Aromatic residues cluster in the core of folded proteins, where they stabilize the structure through multiple interactions. NMR studies in the 1970s demonstrated that aromatic side chains can undergo ring flips—that is, 180° rotations of the χ2 dihedral angle (Cβ–Cγ axis)—even when engaged in stabilizing interactions in the hydrophobic core. Here we capture ring flipping events of a buried tyrosine residue in the SH3 domain of the JNK-interacting protein 1 (JIP1). Our data therefore suggest that the conformation of the aromatic ring at position 526 is determined by steric interactions dictated by the size of the surrounding amino acids.

To study the size correlation between the amino acids at positions 493, 517 and 541 and their influence on the conformation of the aromatic residue at position 526, we carried out a principal component analysis (PCA) by assigning a size score (n) to each amino acid according to the number of heavy atoms in their side chains. This analysis reveals two well-separated groups, with the SH3 domain of JIP1 belonging to group 1. We therefore hypothesized that SH3 domains of group 1 have eclipsed conformations, whereas group 2 have staggered conformations. To test our hypothesis, we determined two crystal structures of SH3 domains of the scaffold protein POSH (‘plenty of SH3 domains’), for which the first SH3 domain belongs to group 2 and the fourth SH3 domain belongs to group 1. Consistent with the PCA, the crystal structure of the first SH3 domain of POSH (POSH-SH3-1) shows a staggered conformation of the corresponding tyrosine residue (Y172), which is stabilized by CH–π interactions from L163 (position 517) and T185 (position 541).

> GRRQLPCAKALYNYEGKEPGDLKFSKGDIIILRRQVDENWYHGEVNGIHGFFPTNFVQIIKPL>[4x]MAKKTSSKGKLPPGPTPLPFIGNYLQLNTEQMYNSLMKISERYGPVFTIHLGPRRVV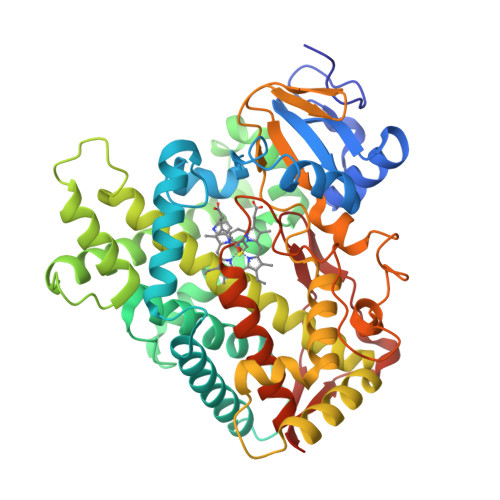VLCGHDAVREALVDQAEEFSGRGEQATFDWVFKGYGVVFSNGERAKQLRRFSIATLRDFGVGKRGIEERIQEEAGFLIDALRGTGGANIDPTFFLSRTVSNVISSIVFGDRFDYKDKEFLSLLRMMLGIFQFTSTSTGQLYEMFSSVMKHLPGPQQQAFQLLQGLEDFIAKKVEHNQRTLDPNSPRDFIDSFLIRMQEEEKNPNTEFYLKNLVMTTLNLFIGGTETVSTTLRYGFLLLMKHPEVEAKVHEEIDRVIGKNRQPKFEDRAKMPYMEAVIHEIQRFGDVIPMSLARRVKKDTKFRDFFLPKGTEVYPMLGSVLRDPSFFSNPQDFNPQHFLNEKGQFKKSDAFVPFSIGKRNCFGEGLARMELFLFFTTVMQNFRLKSSQSPKDIDVSPKHVGFATIPRNYTMSFLPRHHHH> GMQEHYQPAAIEPAAQKKWDDARISNVSEDASKPKYYCLSMFPYPSGKLHMGHVRNYTIGDVLSRFKLLNGFNVMQPMGWDAFGMPAENAAMKNNVAPAAWTYDNIEYMKTQLKSLGFAVDWEREVATCKPEYYRWEQWLFTKLFEKGIVYRKNGTVNWDPVDQTVLANEQVIDGRGWRSGALIEKREIPMYYFKITDYAEELLNDLDKLEHWPEQVKTMQRNWIGKSRGMTVRFAVSDDSKQGLEGDYAKFLQVYTTRPDTLMGATYVAVAAEHPLATAAAADKPELQAFIAECKAGSVAEADMATMEKKGVPTGRYVVNPLNGDKLEVWIANYVLWGYGDGAVMAVPAHDERDFEFAAKYNLPKKQVIAVGDNAFDANRWQEWYGDKENGVLVNSGDLDGLDFQTAFDAVAAKLQSQGAGEPKTQYRLRDWGISRQRYWGCPIPIVHCEKCGNVPVPADQLPVVLPENVVPDGMGSPLAKMPEFYETSCPCCGGAAKRETDTMDTFIESSWYFFRYMSPKFSDGMVSAESAKYWGAVDQYIGGIEHAIGHLLYARFFTKLMRDEGLVNVDEPFERLLTQGMVVCETYYRENDKGGKDWINPADVELTFDDKGRPVSAVLKADGLPVVISGTEKMSKSKNNGVDPQELINAYGADTARLFMMFAAPPEQSLEWSDSGVEGAHRFLRRLWRTVYEYLKQGGAVKAFAGNQDGLSKELKDLRHKLHSTTAKVSDDYGRRQQFNTAIAAVMELLNQYDKTDTGSEQGRAVAQEVLEAAVRLLWPIVPHICETLWSELNGAKLWEAGWPTVDEAALVKSEIEVMVQVNGKLRGKITVAADASKADLEAAALANEGAVKFMEGKPAKKIIVVPGRLVNIVV

To correctly aminoacylate tRNALeu, leucyl-tRNA synthetase (LeuRS) catalyzes three reactions: activation of leucine by ATP to form leucyl-adenylate (Leu-AMP), transfer of this amino acid to tRNALeu and post-transfer editing of any mischarged product. Mechanistically similar to other adenylate-forming enzymes, the class Ia aminoacyl-tRNA synthetase (aaRS) LeuRS charges tRNALeu isoacceptors, which are essential substrates for protein translation. We have solved crystal structures for all enzymatic states of Neisseria gonorrhoeae LeuRS during Leu-AMP formation.

To understand the role of this peptide-plane flip on the global conformational changes and its effects on enzymatic catalysis, L550 was mutated to an alanine or glycine and the crystallization of both mutants was performed. These mutants gave rise to the same crystal form as the WT protein by seeding. However, while the NgLeuRS-L550A diffracted as well as WT protein crystals, the NgLeuRS-L550G showed slightly lower diffraction quality in the range of 2.7–3.3 Å. Comparison of the captured apo and pre-transition states of both mutants show the same large domain movement, including closure of the active site by the CP1 hairpin and structurally associated α-helix (M84-N93), that were seen for the WT structures. Despite the occurrence of these substrate-induced changes, including the shift of the priming loop, no peptide-plane flip was observed in either mutant pre-transition state structure. To further investigate the catalytic role of the L550 peptide-plane flip, the NgLeuRS-L550G mutant was tested for Leu-tRNALeu formation under steady-state (multi-turnover) conditions. A 25-fold decrease in the aminoacylation rate constant was observed (5.8 s−1 vs 0.26 s−1) indicating an important role of the peptide-plane flip in LeuRS turnover. In the first assay NgLeuRS-L550G showed only a twofold decrease in the kcat/KM for Leu activation relative to the WT protein. The transient kinetic analysis unambiguously demonstrated a kinetic defect manifested as a 31-fold drop in the single-turnover rate constants for L550G mutant as compared with WT NgLeuRS (1.7 s−1 vs 52 s−1).>[4x]GMTSPSIESGARERTRRAILDAAMLVLADHPTAALGDIAAAAGVGRSTVHRYYPERTDLLRALARHVHDLSNAAIERADPTSGPVDAALRR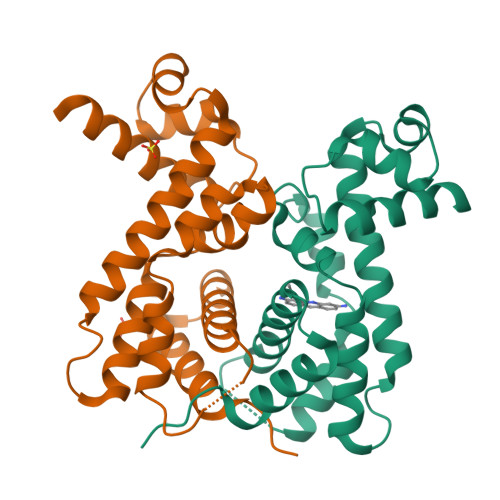VVESQLDLGPIVLFVYYEPSILADPELAAYFDIGDEAIVEVLNRASTERPEYPPGWARRVFWALMQAGYEAAKDGMPRHQIVDAIMTSLTSGIITLPRT> CCGCAGCCTGTACGGACA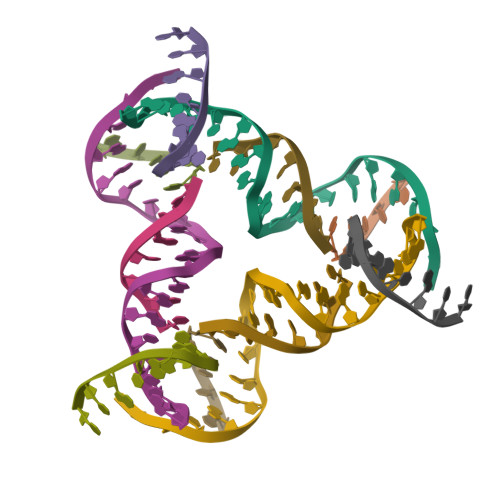TCA;> CCGTACA;> GGCTG;> CCGTGATGT>[2x]DADKLPHTKVTLVAPPQVHPHEQATKSGPKVVEFTMTIEEKKMVIDDKGTTLQAMTFNGSMPGPTLVVHEGDYVQLTLVNPATNAMPHNVDFHGATGALGGAKLTNVNPGEQATLRFKADRSGTFVYHCAPEGMVPWHVVSGMSGTLMVLPRDGLKDPQGKPLHYDRAYTIGEFDLYIPKGPDGKYKDYATLAESYGDTVQVMRTLTPSHIVFNGKVGALTGANALTAK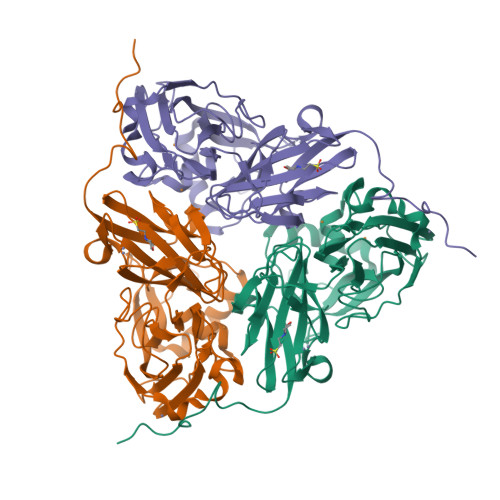VGETVLLIHSQANRDTRPHLIGGHGDWVWETGKFANPPQRDLETWFIRGGSAGAALYTFKQPGVYAYLNHNLIEACELGAAGHIKVEGKWNDDLMKQIKAPAPIPR>MSLRKEPYLLVFGASVVDVFGFSKASYRPYNS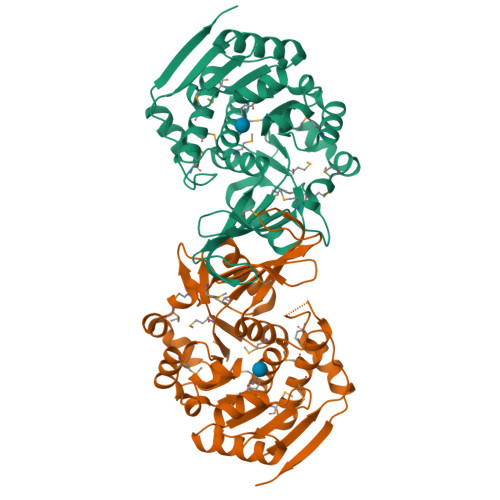TPGHVKISFGGVCRNIAENMARVGVNTNFMSILGNDEHGKSIVEHSKKIGYHMDDSMVIEGGSTPTYLAILDENGEMVSAIADMKSIGAMNTDFIDSKREIFENAEYTVLDSDNPEIMEYLLKNFKDKTNFILDPVSAEKASWVKHLIKDFHTIKPNRHEAEILAGFPITDTDDLIKASNYFLGLGIKKVFISLDADGIFYNDGVSCGKIKATEVDVKNVTGAGDSFVAGLGYGYMNKMPIEDIVKFAMTMSNITISHEETIHPDMALDTVLAKLEKTTWEEEKYDLNEGHHHHHH[2x]>MMSGAPSATQPATAETQHIADQVRSQLEEKYNKKFPVFKAVSFKSQVVAGTNYFIKVHVGDEDFVHLRVFQSLPHENKSL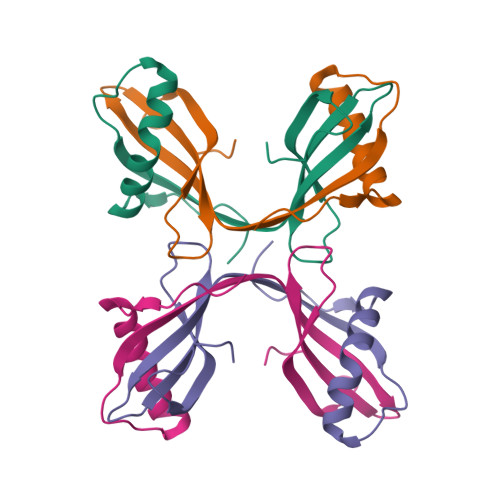TLSNYQTNKAKHDELTYF[2x]> MKTRKLTNILSKLIDKTMAGTSKITDFTPGSASRSLLEAVSLEIEQFYILTKENIDWGIQEGIIEAFDFQKRQSKRAYGDVTIQFYQPLDMRMYIPAGTTFTSTRQEYPQQFETL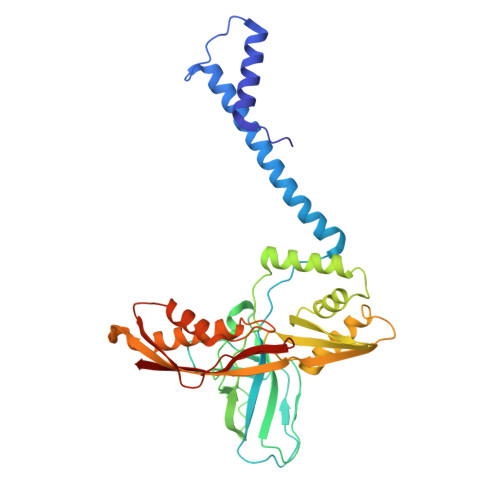VDYYAEPDSTEIVVEVYCKETGVAGNVPEGTINTIASGSSLIRSVNNEYSFNTGTKEESQEDFKRRFHSFVESRGRATNKSVRYGALQIPDVEGVYVYEETGHITVFAHDRNGNLSDTLKEDIIDALQDYRPSGIMLDVTGVEKEEVNVSATVTISNKSRIGDTLQKHIESVIRSYLNNLKTSDDLIITDLIQAIMNIDDVLIYDVSFDNLDENIIVPPQGIIRAGEIKVELK hexane-1,1-diol | C6 H14 O2 | 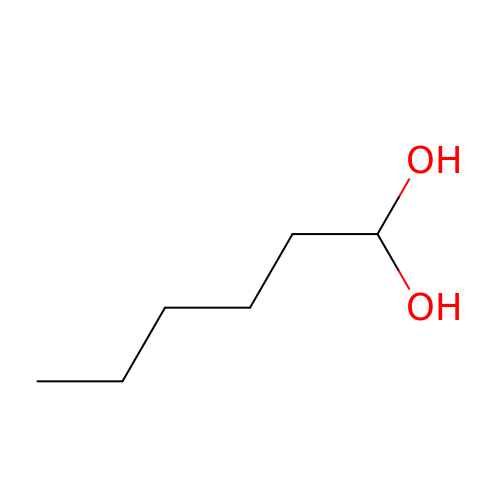ACCCMOQWYVYDOT-UHFFFAOYSA-N> MSHHH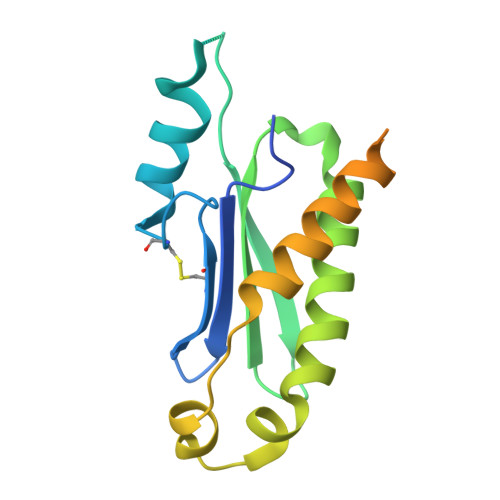HHHSMVDFFTIFSKGGLVLWCFQGVSDSCTGPVNALIRSVLLQERGGNNSFTHEALTLKYKLDNQFELVFVVGFQKILTLTYVDKLIDDVHRLFRDKYRTEIQQQSALSLLNGTFDFQNDFLRLLREAEESSKIRAPTTMKKFEDSEKAKKPVRSMIETRGEKPKEKAKNSKKKGAKKEG> GPNLFVALYDFESRT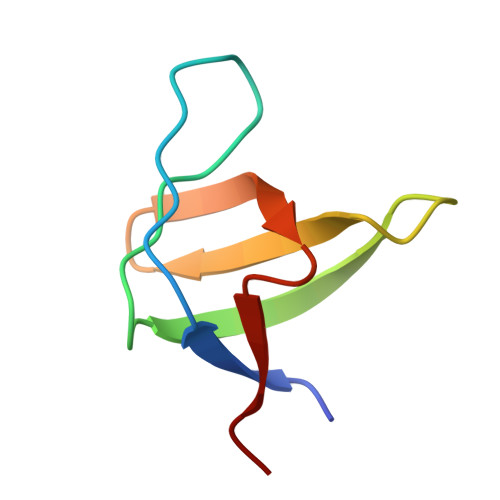ENTLSITKGEKLRVLNNTENGEWCEAQTKNGQGWVPSNYITPVN>MAVRFQKAMETKYTKEWGSNKNKGGKITDKKAKYLRLGYQQNPRKVEMAKCGAAITKKRGLQAYDPKLHLAGIPMGQRQLTPYTISGTDIVCDGDDLHFVNNAAMQQEWDDIRRSCVVGLDLAHEVLEKRLGKEVTPETINYYLEVLNHAMPGAAIVQEHMVETHPALVDDCYVKIFTGDETLQDEVDKQFVINIDNEFPANQAKQIKAAVGKTSWQAVHIPTIVTRTEDGPGTSRWMAMQVGMTFISAYHMCAGEAAVGELAFTAKHAGLVEMGDMIPARRARGPNEPGGLSFGHMADICQTNRKGPEDPVNVILQTASAATMLYDQIWLGGYMSGGVGFTMYATPAYTNDIVDDFLYWADEYASKKYGGRGKAKATIDTVKDIATESTLYSLEAYEKYPTTLEDHFGGSQRATVCSIAAGGATALATGHSQAGLSAWYLSMYLHKEAHGRLGFFGYDLQDQCGATNVFSIASDEGCIGECRGANYPNYAMNVGHQGGYTSVVAAAHAGKDAFCVNPLVKVCFADELINFDFADPRGAFGKAALREWDRCAGERAFVIPAK[2x];>[2x]MADTIDLYSDRGAKLKSGVDINDISPMRNAAIKSIVTGIKRTAAVDLAGIEKTLATSAIGGKGRKIPGREMKLDIVKNAAAIQKAVTEMVQVDSGDDTVVKALNGGKQLIVQVPSVRIDVAAEYVSSLTCTASAVTQALVSQFNIGMFDAPTVKSAVWGQYPQTLDMVGGNVKSIVEIPQKDEGFGYTLRNVMANHLAAVCKKNAMNTAALCSILENTGVFEMGDAIGNQTRHRLLAFSHQGLNANNMVYGTTKALGKTGTIGSAVHACVEKAIADKVISADKKFASGYTTYKTNDVGKWNAYCAAGTLVATLINCGAQRAPQAVSSVLLYFQDLIEKETSLPGCDFGKVQGAAVGFSFFSHSIYGGGGPGVFNGNHVVTRHSKGLAVPCVAAAVALDAGVQVYSPEKTSGLVGDVFSAVDEFREPIKAVAGAV;>[2x]MAYKPQYYPGSTSVAKNRRKFMSDDVEKMRDISDEDLTALLGHRAPGSDYPSTHPPLSEIGEPACPVREVVEPTPGAAAGDRMRYVQFADSMYNGPAVPYWRSYHAAINFRGVDPGTLSGRQVNEMRERDMEEYAKRQSETEITDWGLAGMRGCTVHGXSLRLQEDGVMFDMLDRRRLEGGVIVSDKDQVGVPIDRKVNLGKPMSEAEAAKRTTIYRVDNVAFRSDKEVIEHVQRVWELRTKYGFVPKA

Here, we obtained the true atomic resolution structure of their methane-capturing system (Methyl-Coenzyme M Reductase, MCR), circumventing the isolation barrier by exploiting microbial enrichments of freshwater nitrate-reducing ANME-2d grown in bioreactors, and marine ANME-2c in syntrophy with bacterial partners. Methane capture, the first reaction in AOM, has been proposed to be carried out by the Methyl-Coenzyme M Reductase (MCR). In the proposed mechanism, the heterodisulfide, made of Coenzyme M (HS-CoM) and Coenzyme B (CoB-SH), would react with methane to generate methyl-S-CoM and free CoB-SH through a radical mechanism catalysed by the Ni-containing tetrapyrrole cofactor F43019,20. Despite their physiological differences, these ANMEs have extremely conserved MCR structures, similar to homologs from methanogenic Methanosarcinales, rather than the phylogenetically distant MCR of ANME-1 isolated from Black Sea mats.

Biological samples were retrieved from Ooijpolder (Netherlands)31,32 and Vercelli rice fields (Italy)14,17 and cultivated in bioreactors for >5 years, significantly enriching ANME-2d with nitrate as an electron acceptor. X-ray crystal structures were solved for MCR from ANME-2dO and ANME-2dV, and models were refined to a final resolution of 0.98 Å. Both MCRs crystallised in a monoclinic space group with similar unit cell dimensions. The subatomic resolution of both ANME-2d structures enables the visualisation of the majority of hydrogen atoms and accurately depicts the position of each ligand atom. MCRs from ANME-2c and ANME-2dO contain reduced coenzymes trapped in the active site (i.e. CoM-SH and CoB-SH). In both ANME-2d, a canonical glutamine (position α341 in ANME-2c), proposed to be important to anchor the F430, and juxtaposed to the tyrosine coordinating the CoM thiol (position α342 in ANME-2c), is substituted by a methionine (positions α343 and α347 in ANME-2dO and ANME-2dV, respectively). The substitution does not impact the F430 position and provokes few steric displacements in the vicinity. The three studied enzymes have seven post-translational modifications, among them was a novel 3(S)-methylhistidine on the γ-chain of both ANME-2d MCRs. To our knowledge, this is the first report of a 3(S)-methylhistidine in a natural protein and the first PTM identified on the γ-chain of any characterised MCR. The location of the 3(S)-methylhistidine interacting directly with F430 suggests a compensation for the lack of the methylglutamine in ANME-2dO and ANME-2dV placed in a close proximity.>[2x]MRGSHHHHHHTDPALRALIRVEIPIDAPGIDALLRRSFESDAEAKLVHDLREDGFLTLGLVATDDEGQVIGYVAFSPVDVQGEDLQWVGMAPLAVDEKYRGQGL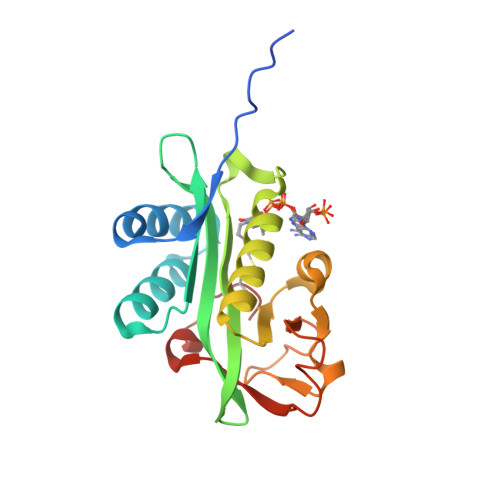ARQLVYEGLDSLNEFGYAAVVTLGDPALYSRFGFELAAHHDLRCRWPGTESAFQVHRLADDALNGVTGLVEYHEHFNRFGLCGR DHOase catalyzes the cyclization of N-carbamoyl-L-aspartate (CA-asp) to L-dihydroorotate (DHO) in the third step of de novo pyrimidine biosynthesis. In mammals, DHOase is a part of a single trifunctional polypeptide of 240 kDa, namely carbamoyl phosphate synthetase (CPSase)/aspartate transcarbamoylase (ATCase)/DHOase protein (CAD), that selfassembles into a hexamer of 1.5 MDa. Almost all of these enzymes contain a similar binuclear metal center consisting of four His, one Asp, and one post-translational carbamylated Lys (Kcx) residue. A further structural study of EcDHOase indicated that a flexible, dynamic loop is extended towards the active site or moved away from the active site when CA-asp is either bound to (loop-in mode) or moved away from the active site (loop-out mode).

For the huDHOase–5-FU complex, the crystals were grown in 0.1 M MES, 1.6 M potassium sodium tartrate tetrahydrate, and 200 μM of 5-FU at pH 6.5. In order to investigate the binding mode, we solved the complexed crystal structure with 5-FU at a 1.97 Å resolution. The two metal ions and the R1475, N1505, T1562, R1661, D1686, H1690, and G1703 residues were involved in 5-FU binding. Similar to the malate binding, 5-FU can bind to huDHOase via the loop-in mode. When compared with apo-huDHOase, the dynamic loop in the huDHOase–5-FU complex was shifted by a distance of 10.2 Å and an angle of 40.4o for 5-FU binding. Even though 5-FU is a nonsubstrate ligand for huDHOase, the flexible loop still did not move away from the active site. Additionally, R1661 and G1703 in huDHOase also interacted with 5-FU through water-molecule-mediated hydrogen bonding. As determined through the titration curve, the Kd value of huDHOase bound to 5-FU was 91.2 ± 1.7 μM. The Kd values of T1562A and R1475A bound to 5-FU were reduced to 146.5 ± 2.1 and 161.5 ± 1.6 μM, respectively. Mutational and structural analyses indicated that the 5-FU binding mode of huDHOase differed from ScDHOase and PaDHPase.

> MTSQKLVRLPGLIDVHVHLREPGGTHKEDFASGTAAALAGGITMVCAMPNTRPPIIDAPALALAQKLAEAGARCDFALFLGASSENAGTLGTVAGSAAGLKLYLNETFSELRLDSVVQWMEHFETWPSHLPIVAHAEQQTVAAVLMVAQLTQRSVHICHVARKEEILLIKAAKARGLPVTCEVAPHHLFLSHDDLERLGPGKGEVRPELGSRQDVEALWENMAVIDCFASDHAPHTLEEKCGSRPPPGFPGLETMLPLLLTAVSEGRLSLDDLLQRLHHNPRRIFHLPPQEDTYVEVDLEHEWTIPSHMPFSKAHWTPFEGQKVKGTVRRVVLRGEVAYIDGQVLVPPGYGQDVRKWPQGAVPQLPPSAPATSEMTTTPERPRRGIPGLPD>[2x]SFTMSGGFELQPRDGGPRVALAPGETVIGRGPLLGITDKRVSRRHAILEVAGGQLR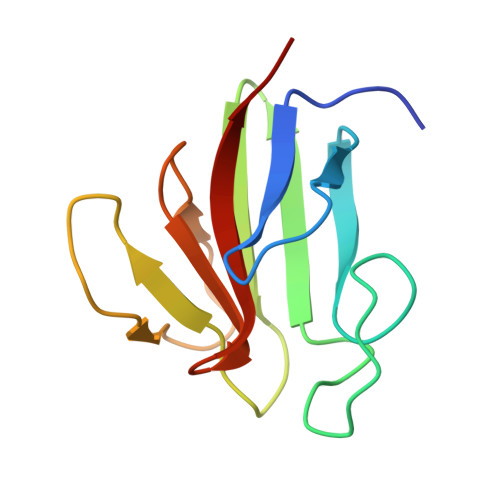IKPIHTNPCFYQSSEKSQLLPLKPNLWCYLNPGDSFSLLVDKYIFRILSIPS Mycobacterium tuberculosis, the causative pathogen of tuberculosis (TB), has three HigBA type II TA systems with reverse gene organization, consisting of the toxin protein HigB and labile antitoxin protein HigA. We studied the MtHigA3 type II TA system protein, a cognate antitoxin of the MtHigB3 ribonuclease toxin. MtHigA3 is predicted to be a transcriptional regulator that autoregulates the higBA3 operon by binding to the operator as an antitoxin itself or via complex formation with the toxin MtHigB3, similar to other type II TA systems. The MtHigA3 antitoxin structure is a homodimer that contains a structurally well conserved DNA-binding domain at the N-terminus and a dimerization domain at the C-terminus.

MtHigA3 bound to DNA was found to crystallize in space group C2 with the MtHigA3 homodimer and 20 bp dsDNA in the asymmetric unit. The electron-density map of the N-terminal 35 amino acids of MtHigA3 bound to DNA was missing, probably due to protease activity. The whole topology of MtHigA3 bound to DNA is similar to that of the MtHigA3 dimer. The overall structures of the MtHigA3 dimer and MtHigA3 bound to DNA are very similar (0.81 Å r.m.s.d. for 78 corresponding Cα atoms of chain A) [Fig. 4(a)]. The interactions between DNA and the MtHigA3 dimer occur mainly through HTH motifs. The recognition α3-helix is inserted in the major groove, and the α2 and the loop that links the α2- and α3-helices support the contacts with the DNA backbone. Interestingly, unusual bending of DNA was observed in MtHigA3 bound to DNA. The DNA fragment bends towards the minor groove with an overall bending angle of 46.5°, as calculated by the CURVES server [Fig. 4(b)]. The average width of the minor groove in canonical B-DNA is 6 Å, but in the structure of MtHigA3 bound to DNA, the width of the minor groove at the A-tract region (bases 9–12) located at the centre of the DNA is narrow (∼3.7 Å). The distance measured from Q64 of each monomer on the α3-helix was increased by 1.9 Å in the MtHigA3 bound to DNA compared with the MtHigA3 dimer (from 37.3 Å to 39.2 Å). The results suggest that rearrangement of the dimer structure is required for DNA binding, providing a wider space between the HTH motifs of each monomer.

>[2x]MTMARNWRDIRADAVAQGRVDLQRAAVAREEMRDAVLAHRLAEIRKALGHARQADVAALMGVSQARVSKLESGDLSHTELGTLQAYVAALGGHLRIVAEFGENTVELTALEHHHHHH>[4x]TQSPALIASQSLWRCTQAHDREGWLALMADDVVIETPIGKSVTNPDGSGIKGKEAVGAFFDTHIAATRLTVTCEET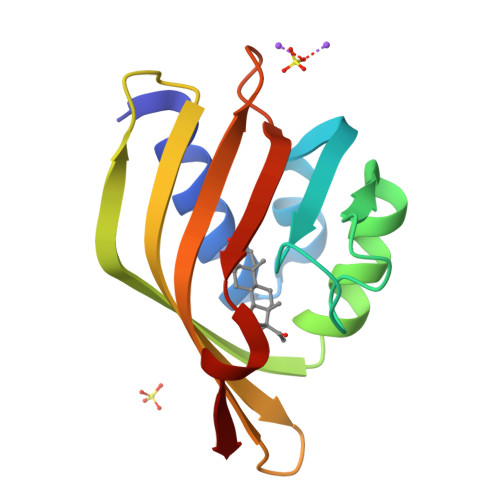FPSSSPDEIAHILVAHSEFDGGFTSEVRGVFTYRVNKAGLITNLRGYWNLDMMTFG> MGSSHHHHHHSSGAGVLTIGCREDSTTFDPIKSAQNRDTWVFANVYDTLVRVDNLGTKMEPGLAESWDISKDGLTYTFKLREAKFSDGSPITAEDAAFSLLRIRD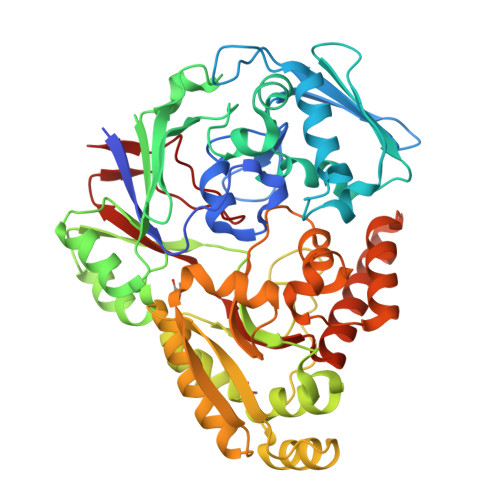NKASLWSDPFSLINTAKATDPKTLVVTLKTPAVAFLSQLASPTVSILSEKAMTKMGEDAYAENPVTSGAFTVDEWRKGDRVILKKNPNFWQAKNVSLDGVEWVSVTDDNTRMRMVQNNELDTAIFVPFSRVEELKKDKNVVIHSDPSTREDHLLINHEHGLLAKPEVRQALDMAIDKQSLVKTATYGQGTVAYSYIPKGSLYHYANNLQRPYDPAAAKKLLADAGAKDLKLNYVVNAGNEADEQIAVIIKDQLAKVGVTANLQKVDPTQSWQMLVDGTYDISVMYWTNDILDPDQKTTFVLGHDTNQNYMTRYKNDQVKALVAAARIEADPAKREQMYIDLQKLAKQDVNWIDLYYSPYINISRKNVSNFLQNPLGRFTLEEVVKN>MQWSGARALEALLTVAGELRGPPLQLDTGQLLKIAKRGGVTAVEAVHAWRNALTGAPLNLTPEQVVAIASHDGGKQALETVQRLLPVLCQAHGLTPQQVVAIASHDGGKQALETVQRLLPVLCQAHGLTPEQVVAIASHDGGKQALETVQALLPVLCQAHGLTPEQVVAIASNGGGKQALETVQRLLPVLCQAHGLTPQQVVAIASNGGGKQALETVQRLLPVLCQAHGLTPQQVVAIASNGGGKQALETVQRLLPVLCQAHGLTPQQVVAIASNNGGKQALETVQRLLPVLCQAHGLTPQQVVAIASNGGGKQALETVQRLLPVLCQAHGLTPQQVVAIASNNGGKQALETVQRLLPVLCQAHGLTPEQVVAIASNGGGKQALETVQRLLPVLCQAHGLTPEQVVAIASHDGGKQALETVQRLLPVLCQAHGLTPQQVVAIASNGGGRPALESIVAQLSRPDPALAALTN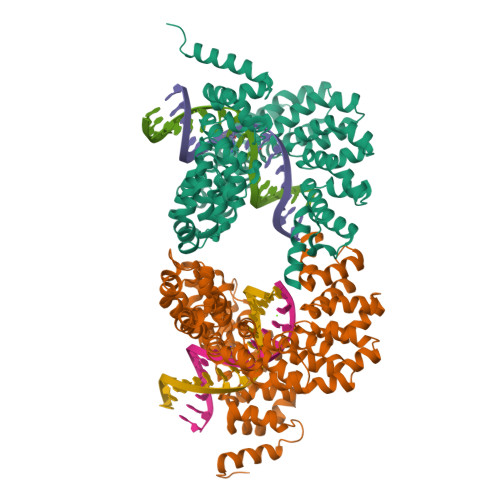DHLVALACLGGRPALDAVKKLEHHHHHH[2x]>GLYFPQRLYTENIYVGQQQGSPLLQVISMREFPTERPYFFLCSHRDAFTSWFHIDEASGVLYLNKTLEWSDFSSLRSGSVRSPKDLTLKVGVSSTPPMKVMCTILPTVEVKLSFINDTAPSCGQVELSTLCFPEKISNPHITENREPGALRQLRRFTHMSICPNYTISYGVVAGSSVPFAVDDSTSELVVTAQVDREEKEVYHLDIVCMVRTERNLEEVFRSLHVNIYDEDDNSPYVNGTDTEDVLVEFDRSEGTVFGTLFVYDRDTTPVYPTNQVQNKLVGTLMTNDSWIKNNFAIEHKFREEKAIFGNVRGTVHEYKLKLSQNLSVTEQRSFLLGYLVNDTTFPGPEGTVLLHFNVTVLPVPIRFSNVTYSFTVSQKATTYSQIGKVCVENCQKFKGIDVTYQLEIVDRNIT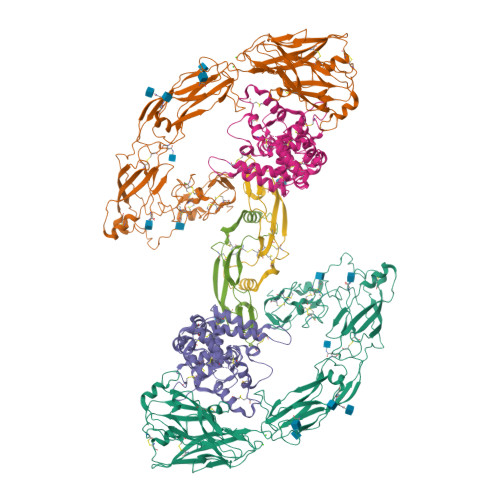AEAQSCYWAVSLAQNPNDNTGVLYVNDTKVLRRPECQELEYVVIAQEQQNKLQAKTQLTVSFQGEADSLRTDEPRFPACAEKRQRGDCEATRGLGAPTGRCQWRQGRDKGISKRYSTCSPNLGTCPDGYCDAIESKNISICPQDCSSEAIIGGYERDLYGIKAGHGTCYCFEGKCFCERDEPEDDICNDMCGSEFENLYFQ[2x];>[2x]EESYFSSSNRLDCVKANELCLKEPGCSSKYRTMRQCVAGRESNFSMATGMEAKDECRLVLDALKQSPLYNCRCKRGMKKEKNCLRIYWGIYQHLQGNDLLEDSPYEPVNSRLSDIFRLAPIYSGEPALAKENNCLNAAKACNLNDTCKKYRSAYISPCTSRVSTAEVCNKRKCHKALRQFFDKVPPKHSYGMLYCSCPLGDQSACSERRRQTIVPACSYEDKERPNCLTLQVSCKTNYICRSRLADFFTNCQPEPLSLSGCLKENYADCLLSYSGLIGTVMTPNYLRSPKISVSPFCDCSSSGNSKEECDRFTEFFTDNACLRNAIQAFGNGGSEFLEVLFQGPGGGENLYFQ;>VKGQGRGCLLKEIHLNVTDLDLGYRTKEELIFRYCSGPCHDAETNYDKILNNLTHNKKLDKDTPSRTCCRPIAFDDDISFLDDSLEYHTLKKHSAKKCACV[2x]> GLSPEKKKMLKKL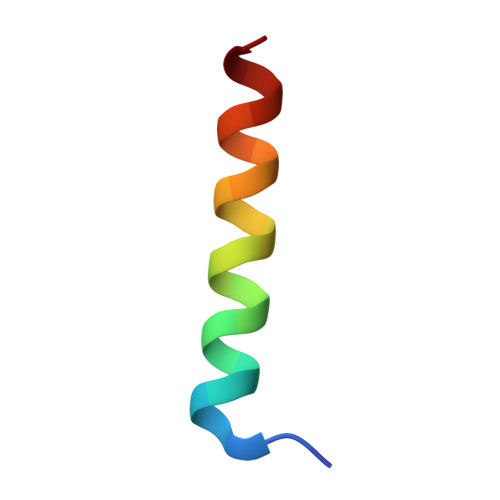IMQKAAEDLAN> MKADNPFDLLLPAAMAKVAEEAGVYKATKHPLKTFYLAITAGVFISIAFVFYITATTGTGTMPFGMAKLVGGICFSLGLILCVVCGADLFTSTVLIVVAKASGRITWGQLAKNWLNVYF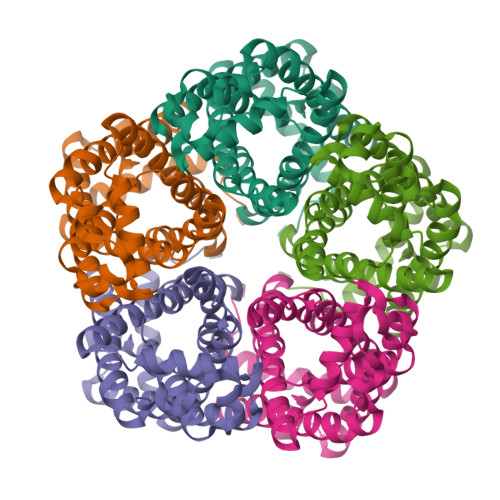GNLVGALLFVLLMWLSGEYMTANGQWGLNVLQTADHKVHHTFIEAVCLGILANLMVCLAVWMSYSGRSLMDKAFIMVLPVAMFVASGFEHSIANMFMIPMGIVIRDFASPEFWTAVGSAPENFSHLTVMNFITDNLIPVTIGNIIGGGLLVGLTYWVIYLRENDHH AMP-activated protein kinase (AMPK) plays an important role in regulating energy homeostasis in eukaryotic cells. AMPK is a heterotrimeric enzyme complex composed of a catalytic α-subunit, together with β- and γ-regulatory subunits. The α-subunit contains an N-terminal protein kinase domain and a C-terminal regulatory domain. The γ-subunit contains four copies of a cystathionine-β-synthase domain27, and we previously showed that the γ-subunit binds three molecules of adenine nucleotide.

The first of these to be reported was A-769662. Initial attempts at co-crystallisation with A-769662 were unsuccessful likely because of the relatively weak binding, poor solubility and the presence of additional, non-specific, binding sites that promote protein aggregation. Utilizing the crystallization conditions for 991, we were able to refine conditions that gave crystals of AMPK in complex with A-769662. Although the diffraction data were limited to 3.9 Å, unbiased electron density maps clearly show that A-769662 is located in the same binding site as 991 and how it overlaps with ring-1 and ring-2 of 991. The two activator complex structures therefore confirm the interpretation of our functional and binding data that A-769662 and 991 activate AMPK through binding to the same site at the interface of the kinase domain and CBM. While there was no CD change upon binding of A-769662, this compound competed for the binding of 991 to AMPK. Together, these data establish that there is a single-binding site common to A-769662 and 991, and likely related compounds. Compound 991 binds about 10-fold tighter than A-769662. Thus, by promoting this CBM/Kinase/regulatory–fragment interaction, 991 and A-769662 enhance protection of the activation loop against dephosphorylation.

>[2x]MSHHHHHHSSGLEVLFQGPMAEKQKHDGRVKIGHYVLGDTLGVGTFGKVKIGEHQLTGHKVAVKILNRQKIRSLDVVGKIKREIQNLKLFRHPHIIKLYQVISTPTDFFMVMEYVSGGELFDYICKHGRVEEMEARRLFQQILSAVDYCHRHMVVHRDLKPENVLLDAHMNAKIADFGLSNMMSDGEFLRTSCGSPNYAAPEVISGRLYAGPEVDIWSCGVILYALLCGTLPFDDEHVPTLFKKIRGGVFYIPEYLNRSVATLLMHMLQVDPLKRATIKDIREHEWFKQDLPSYLFPEDPSYDANVIDDEAVKEVCEKFECTESEVMNSLYSGDPQDQLAVAYHLIIDNRRIMNQASEFYLASSPPSGSFMDDSAMHIPPGLKPHPERMPPLIADSPKARCPLDALNTTKPKSLAVKKAKWHLGIRSQSKPYDIMAEVYRAMKQLDFEWKVVNAYHLRVRRKNPVTGNYVKMSLQLYLVDNRSYLLDFKSIDDEVVEQRSGSSTPQRSCSAAGLHRPRSSFDSTTAESHSLSGSLTGSLTGSTLSSVSPRLGSHTMDFFEMCASLITTLAR;>[2x]MGLNDIFEAQKIEWHEMGNTSSERAALERHGGHKTPRRDSSGGTKDGDRPKILMDSPEDADLFHSEEIKAPEKEEFLAWQHDLEVNDKAPAQARPTVFRWTGGGKEVYLSGSFNNWSKLPLTRSHNNFVAILDLPEGEHQYKFFVDGQWTHDPSEPIVTSQLGTVNNIIQVKKTDFEVFDALMVDSQKCSDVSELSSSPPGPYHQEPYVCKPEERFRAPPILPPHLLQVILNKDTGISCDPALLPEPNHVMLNHLYALSIKDGVMVLSATHRYKKKYVTTLLYKPI;>METVISSDSSPAVENEHPQETPESNNSVYTSFMKSHRCYDLIPTSSKLVVFDTSLQVKKAFFALVTNGVRAAPLWDSKKQSFVGMLTITDFINILHRYYKSALVQIYELEEHKIETWREVYLQDSFKPLVCISPNASLFDAVSSLIRNKIHRLPVIDPESGNTLYILTHKRILKFLKLFITEFPKPEFMSKSLEELQIGTYANIAMVRTTTPVYVALGIFVQHRVSALPVVDEKGRVVDIYSKFDVINLAAEKTYNNLDVSVTKALQHRSHYFEGVLKCYLHETLETIINRLVEAEVHRLVVVDENDVVKGIVSLSDILQALVLTGGEKKP[2x]> MALLGKTLKGRSTRPGGIPQKRNIKWRQLAKNQEEFDQLKQLAKMKREGLKARIKDEQKVVTFNKKKLITYWRKIMRIAKTEQLKNEIDIYSQNNQRELDSKEAFIQMLDKNLDEAEDQFQIALRNHLIHIENLMQLQEARMRGLAEEFNRDVNILETEFDLEREEMVKTHKTQLKELEDMIETVKEEDKKKTEEAQNEFSQFKEETKNKNLEETNVMKIILETKQTKYYTELEQMNSKFQSDTSNKVKDHQFYHAHNKNRKQEIDRYLRTISSKKAKIDLMKLKILQHCKEFNARNSALKKEKENISRNYHELKLKMQKFREEESRRLKELSNNSRNAVLKLREYCALGEKILKTAELCRRLETEKEKVLPFYESSVDEDQIPEQLKNEFEHLKKEDAEEYAYLNNFYKRYNK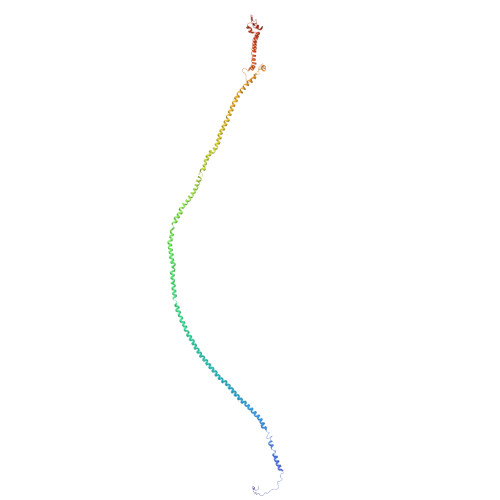VLLDKLAIEKQKENLQRDNQLLKSLLKQYLDGISLNDDVLKNENNPLLVVNHKFNLGKMPVEKIENKTVIEGVFEVRNTSHQLQGQRAPPFQ>[8x]SNAMVDKRESYTKEDLEASGRGELFGAGGPPLPAGNMLMMDRIVKMIEDGGSHNKGYVEAELDINPDLWFFGCHFIGDPVMPGCLGLDAMWQLVG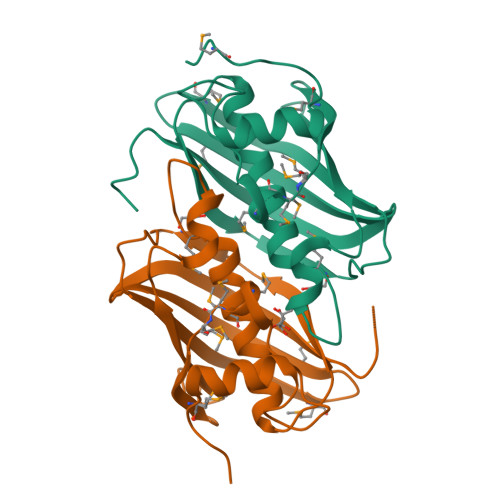FYLGWLGGEGKGRALGVGEVKFTGQVLPDAKKVTYRINFKRVIMRKLIMGVADGEVLVDGKVIYTATDLKVGLFKDTNAF Lanosterol 14α-demethylase (CYP51 or Erg11p in yeast and some fungal pathogens; sterol 14α-demethylase in fungal phytopathogens) is the primary target of the imidazole and triazole (azole) antifungal drugs, often referred to as demethylase inhibitors (DMIs). The CYP51 enzymes of fungal pathogens and yeast use eburicol or lanosterol as substrates to produce ergosterol while their orthologues in plants and humans use obtusifoliol and lanosterol, respectively, to produce plant sterols and cholesterol. In order to better understanding the activity of DMI agrochemicals, we have determined how selected antifungals interact with their target enzyme using S. cerevisiae lanosterol 14α-demethylase as a surrogate. We have also determined seven high resolution X-ray crystal structures of ScErg11p6×His in complex with R- and S-TBZ, R- and S-DPZ, FQZ, PRZ and DFC.

The hydroxyl group of both enantiomers point in the same direction toward Y126 and Y140. S-TBZ binds with its phenylethyl substituent anchored deep in the hydrophobic pocket. The smaller tertiary butyl group of S-TBZ is positioned towards the substrate entry channel. The central quaternary carbons of the enantiomers are approximately 1 Å apart, with R-TBZ projecting deeper into the active site cavity which easily accommodates the smaller tert-butyl substituent. The key water 743 identified in the wild type FLC structure is not seen in either TBZ structure. S-TBZ was found to be the more active enantiomer with 15-fold lower MIC50 than R-TBZ. We observed 8.7 fold (0.64 ± 0.11 μM) and 11.9 fold (0.87 ± 0.06 μM) reduction in susceptibility to S-TBZ in the Y140F and Y140H mutant strains respectively.

> MSATKSIVGEALEYVNIGLSHFLALPLAQRISLIIIIPFIYNIVWQLLYSLRKDRPPLVFYWIPWVGSAVVYGMKPYEFFEECQKKYGDIFSFVLLGRVMTVYLGPKGHEFVFNAKLADVSAEAAYAHLTTPVFGKGVIYDCPNSRLMEQKKFVKGALTKEAFKSYVPLIAEEVYKYFRDSKNFRLNERTTGTIDVMVTQPEMTIFTASRSLLGKEMRAKLDTDFAYLYSDLDKGFTPINFVFPNLPLEHYRKRDHAQKAISGTYMSLIKERRKNNDIQDRDLIDSLMKNSTYKDGVKMTDQEIANLLIGVLMGGQHTSAATSAWILLHLAERPDVQQELYEEQMRVLDGGKKELTYDLLQEMPLLNQTIKETLRMHHPLHSLFRKVMKDMHVPNTSYVIPAGYHVLVSPGYTHLRDEYFPNAHQFNIHRWNNDSASSYSVGEEVDYGFGAISKGVSSPYLPFGGGRHRCIGEHFAYCQLGVLMSIFIRTLKWHYPEGKTVPPPDFTSMVTLPTGPAKIIWEKRNPEQKIGGRHHHHHH(8S)-1,3-dimethyl-8-{[2-(morpholin-4-yl)ethyl]sulfanyl}-6-sulfanylidene-1,3,6,7,8,9-hexahydro-2H-purin-2-one 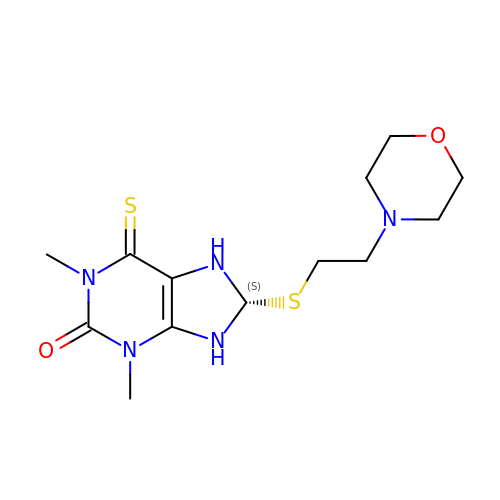| C13 H21 N5 O2 S2 | IDPRQIKRJXLJTP-LBPRGKRZSA-N> GSAMGSASTSGNPFQANVEMKTFMERFNLTHHHQSGIYVDLGQDKEVDGTLYREPAGLCPIWGKHIELQQPDRPPYRNNFLEDVPTEKEYKQSGNPLPGGFNLNFVTPSGQRISPFPMELLEKNSNIKASTDLGRCAEFAFKTVAMDKNNKATKYRYPFVYDSKKRLCHILYVSMQLMEGKKYCSVKGEPPDLTWYCFKPRKSVTENHHLIYGSAYVGENPDAFISKCPNQALRGYRFGVWKKGRCLDYTELTDTVIERVESKAQCWVKTFENDGVASDQPGSGSGSGDQPHSGGVGRNYGFYYVDTTGEGKCALSDQVPDCLVSDSAAVSYTAAGSLSEETPNFIIPSNPSVTPPTPETALQCTADKFPDSFGACDVQACKRQKTSCVGGQIQSTSVDCTADEQNECGSNTAAALVPR

Supporting these invasion events are binary complexes formed between the apical membrane antigen (AMA) and rhoptry neck protein 2 (RON2) families that anchor the junction between parasite and host cell. Specifically, RON2s are transmembrane proteins secreted by apicomplexans into the host cell, integrated into the outer membrane, and presented on the host cell surface to serve as ligands for AMA proteins on the parasite surface. Toxoplasma gondii AMA1 adopts a stacked three domain architecture, with Domain I (DI) membrane distal and Domain III (DIII) membrane proximal. The apical surface is comprised of several loops from DI framing an apical groove, and a single extended loop from DII (DII loop) that packs against the side of DI and is stabilized by three tryptophan anchors buried into pockets on the TgAMA1 apical surface.

Previous structural characterization of TgAMA1 in complex with a RON2 peptide (TgRON2D3) revealed that in order for RON2 to access the TgAMA1 apical groove, the groove-occluding DII loop must be displaced. To probe the role of the DII loop, we engineered a construct of TgAMA1 with the twenty residue mobile portion of the DII loop replaced with a shortened Gly-Ser linker (TgAMA1ΔDIIloop). This engineered construct of TgAMA1 was produced in insect cells, purified, crystallized, and the apo crystal structure solved to 1.93 Å resolution. Superposition of TgAMA1ΔDIIloop on RON2-bound TgAMA1 resulted in a root mean square deviation (rmsd) of 0.70 Å over 365 Cα, indicating strong structural conservation of the protein core. Importantly, a comparison of the apical loops that frame the length of the ligand binding groove showed a maximum deviation of 0.91 Å with an average rmsd of 0.35 Å over 13 to 21 Cαs for the six DI loops indicating that minimal displacement of these loops in TgAMA1ΔDIIloop is necessary for ligand coordination. Overall, truncation of the DII loop in TgAMA1ΔDIIloop appears to faithfully mimic the displaced DII loop form of TgAMA1 and thereby present a mature ligand binding groove. Intriguingly, TgAMA1ΔDIIloop displayed notably different binding profiles compared to TgAMA1, aside from a similar affinity for the cognate ligand, TgRON2D3. In addition, binding was detected between TgAMA1ΔDIIloop and TgRON2L2D3, TgRON2L1D3 and PfRON2D3 in the micromolar range (6.0, 46, and 1.4 μM, respectively). Collectively, these results suggest that while the TgAMA1 groove is fundamentally capable of interacting with all the RON2D3 peptides tested, the presence of the DII loop imparts remarkable selectivity. However, since the presence of the AMA1 DII loop results in a more selective receptor, this substructure may act as a structural gatekeeper to restrict formation of unproductive AMA1 complexes.> X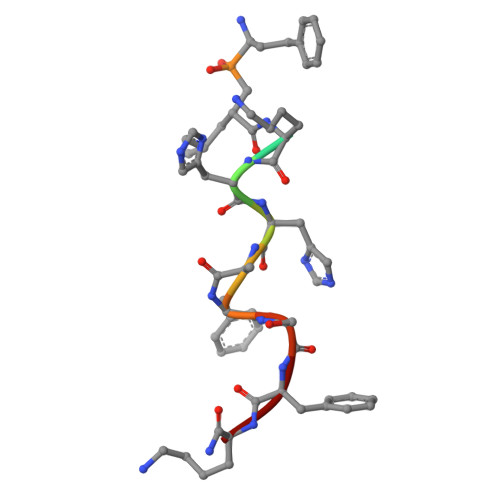XKHHAFSFK>[2x]MSAPTPLAEASQIPTIPALSPLTAKQSKGNFFSSNPISS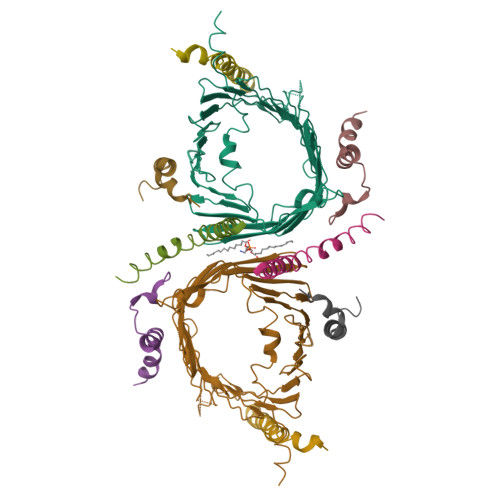FVVDTYKQLHSHRQSLELVNPGTVENLNKEVSRDVFLSQYFFTGLRADLNKAFSMNPAFQTSHTFSIGSQALPKYAFSALFANDNLFAQGNIDNDLSVSGRLNYGWDKKNISKVNLQISDGQPTMCQLEQDYQASDFSVNVKTLNPSFSEKGEFTGVAVASFLQSVTPQLALGLETLYSRTDGSAPGDAGVSYLTRYVSKKQDWIFSGQLQANGALIASLWRKVAQNVEAGIETTLQAGMVPITDPLMGTPIGIQPTVEGSTTIGAKYEYRQSVYRGTLDSNGKVACFLERKVLPTLSVLFCGEIDHFKNDTKIGCGLQFETAGNQELLMLQQGLDADGNPLQALPQL;>MSFLPSFILSDESKERISKILTLTHNVAHYGWIPFVLYLGWAHTSNRPNFLNLLSPLPSV[2x];>[2x]MVELTEIKDDVVQLDEPQFSRNQAIVEEKASATNNDVVDDEDDSDSDFEDEFDENETLLDRIVALKDIVPPGKRQTISNFFGFTSSFVRNAFTKSGNLAWTLTTTALLLGVPLSLSILAEQQLIEMEKTFDLQSDANNILAQGEKDAAATANGSPGHHHHHHHHHH;>MFGLPQQEVSEEEKRAHQEQTEKTLKQAAYVAAFLWVSPMIWHLVKKQWK[2x];>[2x]MDGMFAMPGAAAGAASPQQPKSRFQAFKESPLYTIALNGAFFVAGVAFIQSPLMDMLAPQL[4-oxidanyl-4-(phenylmethyl)piperidin-1-yl]-(2-pyridin-4-ylpyridin-3-yl)methanone | C23 H23 N3 O2 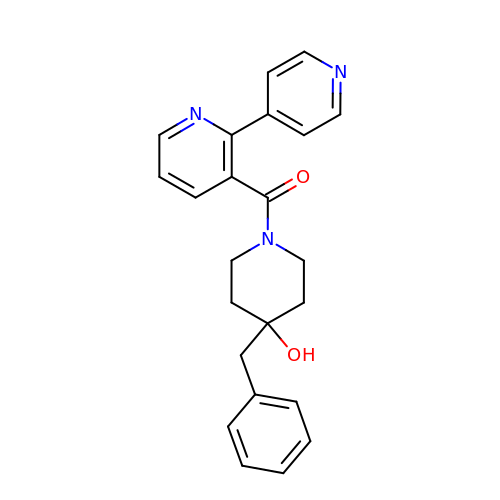| XKUZMIUSBMCVPP-UHFFFAOYSA-N>[18x]MSGFGGGSSGAGSLTQLLATGSMDAALTQNATRTFWKSSYQKHSLFALESINQPFTTQVQFGAESHITVNRQGDLLSWMYLKIVLPGLKVQNQADTVQPTQQSFASLDNDVAAQADVSHVLPYIEGAYTEASLNTKEQLIAEAKNSYEAAKYNAAPLPVAAQMQSTEMPDFDYAYWTEAIGFHLIKRAEFKVGGATIDTIWSELLFAMEELMGRAGRRLTETIGRTLRRPTELMKASRQEQILYVPLPWYFTKHPSLAFPLVAATYHNIQLWVQWAQLNSCIIKSRSNLVVLHAERNVPISDDHLRASLECTYVHLEAAERDALTANAGTQLIVQHQAHLQQVSSNNVTARLNFNFPVLEFYYFLRRKANKDAGDHFNFS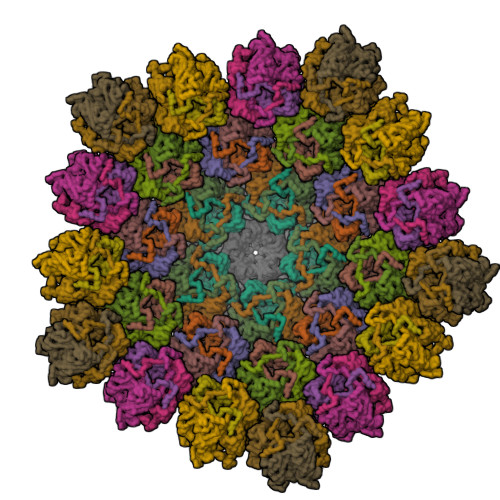GIGGRDPVVSAELLFNNTARVTQKPAVWWRAVQALQFHSSAPLTNIYSYSFSLSPEDPITPSGSANFSRLDSVELALTLQDDFGAAHDANSELFVFARSYNILKFTNGLAGLLYSN;> MPSIAFSGISTKPGELEFHVPSVLSKHNRAGLLKSIDFPYSQRTIESSWNKLHYMESIRITPESRSVSVLLTDKESGDRVEMLAMVPLTTNKIIEISTATTDGTIILVTEEPHGFFAPGCFGKEVRNVISSYKSIFPHGTPPFILIHGSNGSVQVDPALFEYNDEYSVKIKYTAIRTEFKLFGKGDHGWMVTPEFPTISMLCQVITNAMNSAIIFNHDDPAARTRMYPGTCSNTHVIESVSGDSLAKALLGYDGVYAGWEEITIPAGMYCYGELDLSKMIAAKMNRWHIDRESSIIFRGVSGYTWNVTLPSGNYGTPEKLAHCIQHMMNMTAKNRKNPYCVRFTLNEGSSHRGKFVFVAAEPFDLLFGDDESIDPSILGFEPVDHIGRNSYMSENDLGAPLMKPNCNVYDVDEIPGTHQIRIGRRTRLAVDGKIRGYSGGTLRLNTVNRTTGAPKCHGMNKGDVVTLTTVMPAPDGATGTKREGFTFRAKNKIMGVVVADENENPDASSLHVSVPSMSWTLGIGSYITIDSQAAPISVALFDPGKNQFFRDSIGASRLGFSNGVSTGQHGVVVSQCAVNLEPRTVDVSFIEGSMTSASTEMYNQNGKSLITQVPSDRSSGPVPQGMVRFNNALQQFKLEFTNPDGSPYHFNHASLSLLMEFDD(2~{R},3~{R},4~{S},5~{R})-2-(6-aminopurin-9-yl)-5-[[3-(6-azanyl-9~{H}-purin-8-yl)prop-2-ynyl-methyl-amino]methyl]oxolane-3,4-diol | C19 H21 N11 O3 | 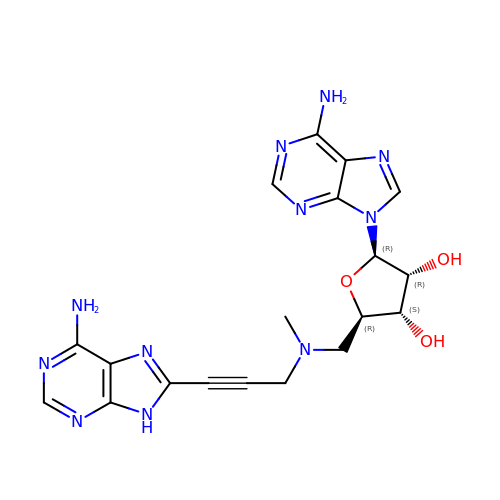MNFDLXSVTTXDGC-NBKUUXFISA-N>[2x]MSTPADRARLLIKKIGPKKVSLHGGDYERWKSVSKGAIRVST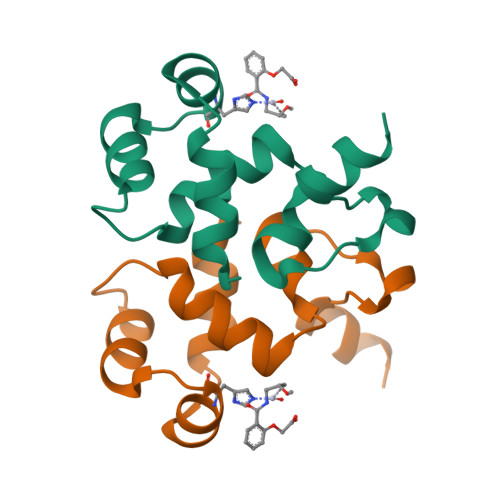EEIDVLVKIFPNYALWIASGSIAPEVGQTSPDYDEANLNLSNQNAGAHHHHHH> AMGNDTYQPINCDDYDNLELACQHHLMLTLE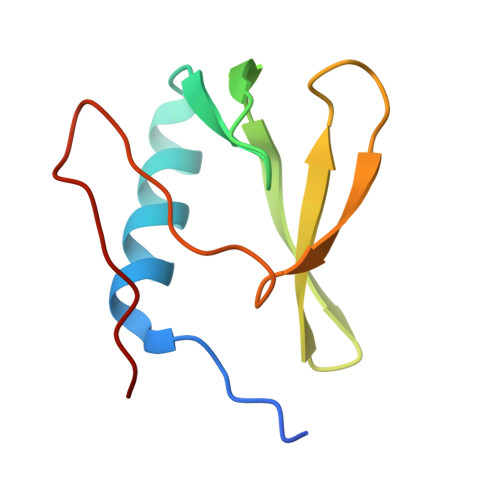LKDGEKLQAKASDLVSRKNVEYLVVEAAGETRELRLDKITSFSHPEIGTVVVSES>[2x]LVPRGSHMNPNYDENSNQAFASATNDIDKNSHD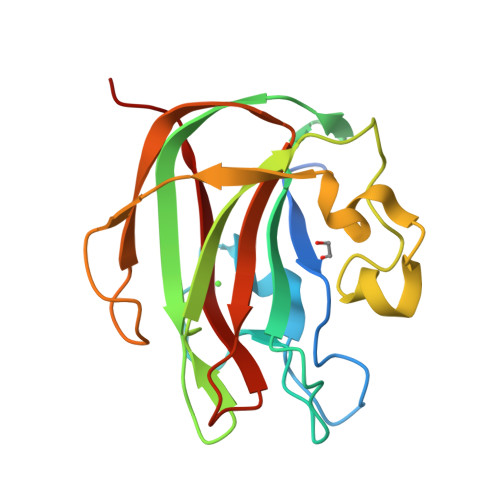RVDYLNDGDHSENRRWTNWSPTPSSNPEVSAGVIFRENGKIVERTVAQAKLHFFADSGTDAPSKLVLERYVGPGFEVPTYYSNYQAYESGHPFNNPENWEAVPYRADKDIAAGDEINVTFKAVKAKAMRWRMERKADKSGVAMIEMTFLAPSE> MVFGQLYALFIFTLSCCISKTVQADSSKESSSFISFDKESNWDTISTISSTADVISSVDSAIAVFEFDNFSLLDNLMIDEEYPFFNRFFANDVSLTVHDDSPLNISQSLSPIMEQFTVDELPESASDLLYEYSLDDKSIVLFKFTSDAYDLKKLDEFIDSCLSFLEDKSGDNLTVVINSLGWAFEDEDGDDEYATEETLSHHDNNKGKEGDDDILSSIWTEGLLMCLIVSALLLFILIVALSWISNL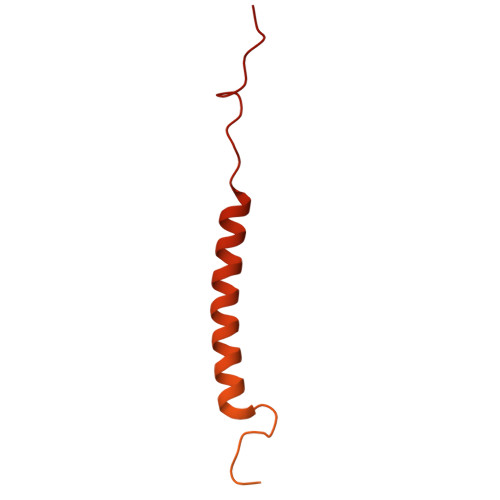DITYGALEKSTNPIKKNN> AAANLRKTCVHRLNSGG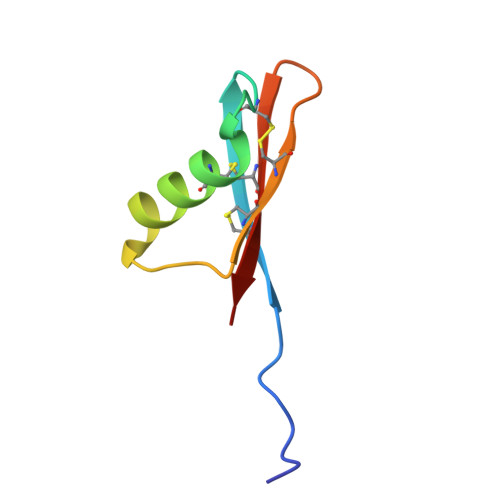SCGKSGQHDCEAFYTNKTNQKAFYCNCTSPFRTRYCDCAIAA> MQTDTSNRLKQIMAERNLKQVDILNLSIPFQKKFGIKLSKSTLSQYVNSVQSPDQNRIYLLAKTLGVSEAWLMGFDVPMVESSK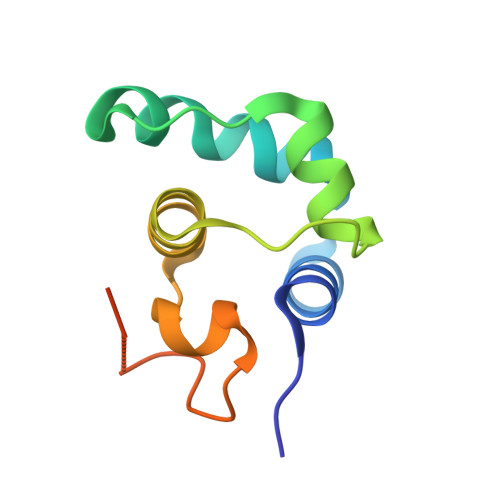IENDSHHHHHH>ATCYCRTGRCATRESLSGVCEIS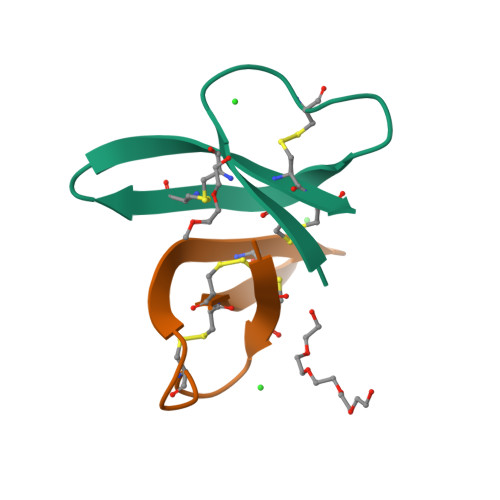GRLYALCCR[6x]Here we report three-dimensional structures of three large ornate bacterial RNAs using cryo-electron microscopy (cryo-EM). GOLLD (Giant, Ornate, Lake- and Lactobacillales-Derived), ROOL (Rumen-Originating, Ornate, Large) and OLE (Ornate Large Extremophilic) RNAs form homo-oligomeric complexes whose stoichiometries are retained at lower concentrations than measured in cells. Unexpectedly, the three structures are stabilized not by proteins but by other copies of the same RNA molecule in ornate quaternary assemblies with many intermolecular bridges, a phenomenon that has not previously been observed for natural RNA molecules. Extensive intramolecular and intermolecular A-minor interactions, kissing loops, an unusual A–A helix and other interactions stabilize the three complexes.

GOLLD RNAs are the largest among the three RNA classes analysed here, with many members exceeding 800 nucleotides in length. The 3D reconstruction at 3.0 Å resolution shows that GOLLD forms a nanocage, similar to the one formed by ROOL, but larger. The GOLLD structure is a closed 14-mer with D7 quaternary symmetry, with a diameter of 380 Å and a completely empty interior except for a disordered loop. Beyond confirming the accuracy of the previously predicted secondary structure with stems P1–P27, the tertiary structure of GOLLD reveals prominent interactions, including A-minor interactions involving adenosines at the P3–P4–P5 junction, an A-minor interaction between adenosines in L26 and stem P14 and a loop L22 that forms a pseudoknot with the nearby linker J17/22, in addition to an A-minor interaction with that pseudoknot. Similar to ROOL, the variable linker within each chain is not resolved, but the positions of immediate flanking sequences in the 5′ and 3′ regions indicate that the linker resides in the interior of the cage. Globally, the cryo-EM structure shows that the 5′ region and the 3′ region form separate domains in the 3D structure. The 5′ domains of GOLLD form the cap of each half-shell of the nanocage. Within the cap of each half-shell, each of 7 monomers forms 8 quaternary bridges to other chains—4 on each side, including kissing loops, A-minor interactions and other interactions (B2–B5). Only a single intermolecular A-minor interaction, B1, glues the 3′ and 5′ regions from different chains together. In the GOLLD nanocage, these interactions consist of two self-interacting kissing-loop interactions (B8 and B9) and an A-minor interaction (B10) involving 3′ regions from different chains.

>GGAUGGCCGCCUAUGGUCGUCAAAUAAACUACGAAAGUAGGAUAAAGUGGAAUAGUAAGGUUUAGCUAUUCUGCGGUUUCAUCUUGUAAAGAUGGAGCUUGAGUAGGCAAGUGAGAUAUCAAUUUUUCUUAGUAUGUGAGGGUAACACUUUAGCAGAGGAGAAAAGUUGACUGGGUCUUUGCAGAGAUUCAGUUGAGUUCGGAAGAGCAAUAAGAAUAACUCAUAGAAUUCAAUGCGAGAGGUAGGGAACUAAUCCCUCCCUAUAAUCGCGGUAUUCAAUAUGAUAGUUUACUUAACAUCAAAUUGGGGAAACCCUUUAAGAUAAGAUAGUGUACGGGUGGUGCCGUUAUUAUCCUUUGAUAGAGUGUACCAGCACCUAUCGAUGAAGUAAACUUGGAAUAUGGUGGUAGGGAUACCACAUCGGGUAGUUAAGUAUUCUGUCGUUCAAAAGGCGGCGGAGCUUGUGAUAGACCGCUACCUGAAACCACUGCAAAACCAAACUUAUAUUUGCAUUUAGGAUUGCAAAAUCAUAAAAAUCAAAAUAAGAAAAAGUGUCUAUCAGUUUUGACCGAAAGGUGUCUACAUAGUAAUGAGUUGUUCAUUGCCACAAACACUCUCAAGGUGAAUGUGAUUCUUUCGAAAGGUUUCUAACACCGCAAGUGUGAAUCUGCUCGGCAGGGUAGAAGAAAAUAAGUAAGAAGAGAGUAGGUUAAAACUCAAAGAGUGGUUCACUUAAAUAACCGACAUUGGUUGUUACAUCUCAAAAGGAUGUGGAAACAAAGGGAAUAGAUAAUCCUUUUAAAGACAACUACAAUAUGGUGUAUUCUCAGCCU[14x]>[2x]MERDGCAGGGSRGGEGGRAPREGPAGNGRDRGRSHAAEAPGDPQAAASLLAPMDVGEEPLEKAARARTAKDPNTYKVLSLVL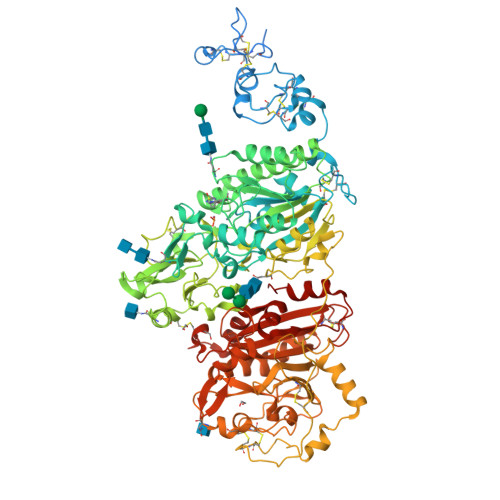SVCVLTTILGCIFGLKPSCAKEVKSCKGRCFERTFGNCRCDAACVELGNCCLDYQETCIEPEHIWTCNKFRCGEKRLTRSLCACSDDCKDKGDCCINYSSVCQGEKSWVEEPCESINEPQCPAGFETPPTLLFSLDGFRAEYLHTWGGLLPVISKLKKCGTYTKNMRPVYPTKTFPNHYSIVTGLYPESHGIIDNKMYDPKMNASFSLKSKEKFNPEWYKGEPIWVTAKYQGLKSGTFFWPGSDVEINGIFPDIYKMYNGSVPFEERILAVLQWLQLPKDERPHFYTLYLEEPDSSGHSYGPVSSEVIKALQRVDGMVGMLMDGLKELNLHRCLNLILISDHGMEQGSCKKYIYLNKYLGDVKNIKVIYGPAARLRPSDVPDKYYSFNYEGIARNLSCREPNQHFKPYLKHFLPKRLHFAKSDRIEPLTFYLDPQWQLALNPSERKYCGSGFHGSDNVFSNMQALFVGYGPGFKHGIEADTFENIEVYNLMCDLLNLTPAPNNGTHGSLNHLLKNPVYTPKHPKEVHPLVQCPFTRNPRDNLGCSCNPSILPIEDFQTQFNLTVAEEKIIKHETLPYGRPRVLQKENTICLLSQHQFMSGYSQDILMPLWTSYTVDRNDSFSTEDFSNCLYQDFRIPLSPVHKCSFYKNNTKVSYGFLSPPQLNKNSSGIYSEALLTTNIVPMYQSFQVIWRYFHDTLLRKYAEERNGVNVVSGPVFDFDYDGRCDSLENLRQKRRVIRNQEILIPTHFFIVLTSCKDTSQTPLHCENLDTLAFILPHRTDNSESCVHGKHDSSWVEELLMLHRARITDVEHITGLSFYQQRKEPVSDILKLKTHLPTFSQED>MNDSNSLLITRLAAQILSRNMQTVDVIVDDKTLSLEEKIDTLTSMVLAVNSPPQSPPRVTSSDLAASIIKNNSKMVGNDFEMRYNVLRMAVVFVKHYPKYYNETTAGLVAEIESNLLQYQNYVNQGNYQNIEGYDSLLNKAEECYVKIDRLFKESIKKIMDDTEAFEREQEAERLRAEQTAANALLERRAQTSADDVVNRADANIPTAFSDPLPGPSAPRYMYESSESDTYMETARRTAEHYTDQDKDYNAAYTADEYNSLVKTVLLRLIEKALATLKNRLHITTIDQLKKFRDYLNSDADAGEFQIFLNQEDCVILKNLSNLASKFFNVRCVADTLEVMLEALRNNIELVQPESDAVRRIVIKMTQEIKDSSTPLYNIAMYKSDYDAIKNKNIKTLFDLYNDRLPINFLDTSATSPVRKTSGKRSAEDDLLPTRSSKRANRPEINVISSEDEQEDDDVEDVDYEKESKRRKLEDEDFLKLKALEFSKDIVNEKLQKIIVVTDGMKRLYEYCNCKNSLETLPSAANYGSLLKRLNLYNLDHIEMNVNFYELLFPLTLYNDNDNSDKTLSHQLVNYIFLASNYFQNCAKNFNYMRETFNVFGPFKQIDFMVMFVIKFNFLCDMRNFAKLIDELVPNKQPNMRIHSVLVMRDKIVKLAFSNLQFQTFSKKDKSRNTKHLQRLIMLMNANYNVI[3x];> MECPFQIQVCISDRFFAFPHNLVEPQSDVGNKLIENLIVYVPTDDDRLYIDKKQFPKFNSVLVYRHEHDVNIDSRSPKKTASATIVYWNPLVPITEIGAGETRVFSVLLTNNLFYCNTMIVHHENPKCPIEFTYPETDMQSACSALLKNRNGQSVPPPIKSNLRPIACEIPLSHFKELVESNDFLLCFNLETSTMVKILSLKRIFCIFQYRKQPARYVINLPHEEIDNLYNKLNWERTRRLMKGDVPSNCATVNRSSLKYIKQAQSLLGIPDYSQTVVDFVKMFQKIIFPYQLVPNVIIKLNNFDQMVSSAPNKAEPYKKIRLFCKNDSIAISSSGIVPINMPDFSPPNTFDYSDYANRTNINFVTQRVLTDGGFSSGITVTPVKYNYYL;> MSGGGNLLTLERDHFKYLFLTSYFDLKDNEHVPSEPMAFIRNYLNCTFDLLDDAVLMNYFNYLQSMQLKHLVGSTSTNIFKFVKPQFRFVCDRTTVDILEFDTRMYIKPGTPVYATNLFTSNPRKMMAFLYAEFGKVFKNKIFVNINNYGCVLAGSAGFLFDDAYVDWNGVRMCAAPRLDNNMHPFRLYLLGEDMAKHFVDNNILPPHPSNAKTRKINNSMFMLKNFYKGLPLFKSKYTVVNSTKIVTRKPNDIFNEIDKELNGNCPFIKFIQRDYIFDAQFPPDLLDLLNEYMTKSSIMKIITKFVIEENPAMSGEMSREIILDRYSVDNYRKLYIKMEITNQFPVMYDHESSYIFVSKDFLQLKGTMNAFYAPKQRILSILAVNRLFGATETIDFHPNLLVYRQSSPPVRLTGDVYVVDKNEKVFLVKHVFSNTVPAYLLIRGDYESSSDLKSLRDLNPWVQNTLLKLLIPDSVQ;>MSAIALYLEINKLRLKIDEPMQLAIWPQLFPLLCDEHQSVQLNTDVLINFMMHVARKSQNTILNNNAAIASQYAAGNADVVAAPASAQPTPRPVINLFARANAAAPAQPSEELINMRRYRNAARKLIHHYSLNSTSSTEYKISDVVMTMIFLLRSEKYHSLFKLLETTFDDYTCRPQMTQVQTDTLLDAVRSLLEMPSTTIDLTTVDIMRSSFARCFNSPIMRYAKIVLLQNVALQRDKRTTLEELLIERGEKIQMLQPQQYINSGTEIPFCDDAEFLNRLLKHIDPYPLSRMYYNAANTMFYTTMENYAVSNCKFNIEDYNNIFKVMENIRKHSNKNSNDQDELNIYLGVQSSNAKRKKY[2x];>MKRIKCNKVRTVTEIVNSDEKIQKTYELAEFDLKNLSSLESYETLKIKLALSKYMAMLSTLEMTQPLLEIFRNKADTRQIAAVVFSTLAFIHNRFHPLVTNFTNKMEFVVTETNDTSIPGEPILFTENEGVLLCSVDRPSIVKMLSREFDTEALVNFENDNCNVRIAKTFGASKRKNTTRSDDYESNKQPNYDMDLSDFSITEVEATQYLTLLLTVEHAYLHYYIFKNYGVFEYCKSLTDHSLFTNKLRSTMSTKTSNLLLSKFKFTIEDFDKINSNSVTSGFNIYNFNK[2x];> MASSLQSKWICLRLNDAIIKRHVLVLSEYADLKYLGFEKYKFFEYVIFQFCNDPQLCKIIENNYNYCMQIFKAPADDMRDIRHNIKRAFKTPVLGHMCVLSNKPPMYSFLKEWFLLPHYKVVSLKSESLTWGFPHVVVFDLDSTLITEEEQVEIRDPFVYDSLQELHEMGCVLVLWSYGSRDHVAHSMRDVDLEGYFDIIISEGSTVQEERSDLVQNSHNAIVDYNLKKRFIENKFVFDIHNHRSDNNIPKSPKIVIKYLSDKNVNFFKSITLVDDLPTNNYAYDFYVKVKRCPTPVQDWEHYHNEIIQNIMDYEQYFIK;>MALVPVGMAPRQMRVNRCIFASIVSFDACITYKSPCSPDAYHDDGWFICNNHLIKRFKMSKMVLPIFDEDDNQFKMTIARHLVGNKERGIKRILIPSATNYQDVFNLNSMMQAEQLIFHLIYNNENAVNTICDNLKYTEGFTSNTQRVIHSVYATTKSILDTTNPNTFCSRVSRDELRFFDVTNARALRGGAGDQLFNNYSGFLQNLIRRAVAPEYLQIDTEELRFRNCATCIIDETGLVASVPDGPELYNPIRSSDIM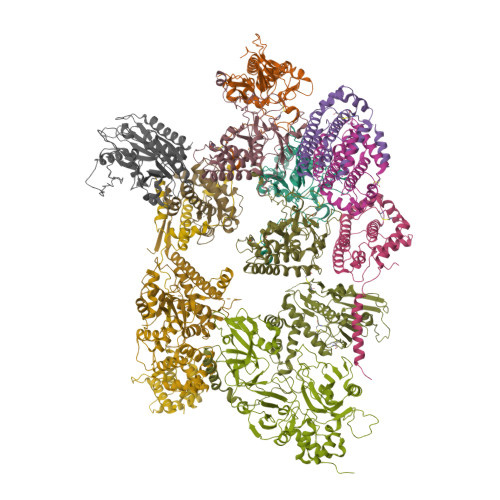RSQPNRLQIRNVLKFEGDTRELDRTLSGYEEYPTYVPLFLGYQIINSENNFLRNDFIPRANPNATLGGGAVAGPAPGVAGEAGGGIAV[4x]> MKQYQDLIKDIFENGYETDDRTGTGTIALFGSKLRWDLTKGFPAVTTKKLAWKACIAELIWFLSGSTNVNDLRLIQHDSLIQGKTVWDENYENQ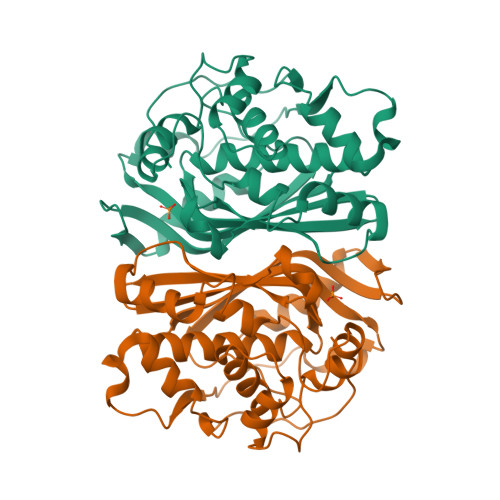AKDLGYHSGELGPIYGKQWRDFGGVDQIIEVIDRIKKLPNDRRQIVSAWNPAELKYMALPPCHMFYQFNVRNGYLDLQWYQRSVDVFLGLPFNIASYATLVHIVAKMCNLIPGDLIFSGGNTHIYMNHVEQCKEILRREPKELCELVISGLPYKFRYLSTKEQLKYVLKLRPKDFVLNNYVSHPPIKGKMAV ENPP1 (Ecto-nucleotide pyrophosphatase phosphodiesterase 1) is a type II transmembrane glycoprotein originally identified as a negative regulator of bone mineralization. ENPP1 is expressed on the cell surface in mineralizing cells, such as osteoblasts and chondrocytes, and hydrolyzes extracellular ATP to produce AMP and diphosphate, an inhibitor of bone mineralization. A recent study reported that ENPP1 also hydrolyzes 2′3′-cGAMP, but not 3′3′-cGAMP, and negatively regulates the cGAS-STING-dependent immune activation. Here, we report the crystal structures of ENPP1 in complex with 3′3′-cGAMP and the reaction intermediate pA(3′,5′)pG (pApG).

We co-crystallized the ENPP1-ΔSMB T238A mutant in the presence of 2′3′-cGAMP or 3′3′-cGAMP, and determined the crystal structures at 1.8 and 1.9 Å resolutions, respectively. In the co-crystal structure with 2′3′-cGAMP, a continuous density was not observed at the 2′-5′ phosphodiester linkage of 2′3′-cGAMP, suggesting that 2′3′-cGAMP was predominantly degraded to the pApG linear intermediate during crystallization, although the catalytically inactive ENPP1-ΔSMB T238A mutant was used for crystallization. This may be due to the slight enzymatic activity of the mutant at a high concentration during crystallization. We concluded that this structure represents a post-reaction state of the first hydrolysis, and modeled pApG into the electron density. pApG adopts an open conformation, in which the nucleobases are far apart from each other. The adenine and guanine moieties of pApG are accommodated within the nucleotide-binding pocket (N-pocket) and the guanine-binding pocket (G-pocket), respectively. The 5′-phosphate group binds to two zinc ions (Zn1 and Zn2), which are coordinated by Asp358/His362/His517 and Asp200/Asp405/His406, respectively. This observation suggests that ENPP1 first hydrolyzes the 2′-5′, rather than the 3′-5′, phosphodiester linkage in 2′3′-cGAMP, consistent with previous data showing that a 2′3′-cGAMP analog with the 2′-5′ non-hydrolyzable phosphothioate diester linkage (2′3′-cGAsMP) is not degraded by ENPP123. The guanosine moiety of pApG is accommodated in the G-pocket, formed by His362 on a short helix and a loop (residues 510–517). The 3′-OH group of the guanosine forms a hydrogen bond with Asn259, while the guanine base is stacked with His362, with its N1 atom forming a hydrogen bond with Ser514.

> GPKSWVEETCESIDTPECPAEFESPPTLLFSLDGFRAEYLHTWGGLLPVISKLKNCGTYTKNMRPMYPTKAFPNHYSIVTGLYPESHGIIDNKMYDPKMNASFSLKSKEKFNPLWYKGQPIWVTANHQEVKSGTYFWPGSDVEIDGILPDIYKVYNGSVPFEERILAVLEWLQLPSHERPHFYTLYLEEPDSSGHSHGPVSSEVIKALQKVDRLVGMLMDGLKDLGLDKCLNLILISDHGMEQGSCKKYVYLNKYLGDVNNVKVVYGPAARLRPTDVPETYYSFNYEALAKNLSCREPNQHFRPYLKPFLPKRLHFAKSDRIEPLTFYLDPQWQLALNPSERKYCGSGFHGSDNLFSNMQALFIGYGPAFKHGAEVDSFENIEVYNLMCDLLGLIPAPNNGSHGSLNHLLKKPIYNPSHPKEEGFLSQCPIKSTSNDLGCTCDPWIVPIKDFEKQLNLTTEDDDIYHMTVPYGRPRILLKQHRVCLLQQQQFLTGYSLDLLMPLWASYTFLSNDQFSRDDFSNCLYQDLRIPLSPVHKCSYYKSNSKLSYGFLTPPRLNRVSNHIYSEALLTSNIVPMYQSFQVIWHYLHDTLLQRYAHERNGINVVSGPVFDFDYDGRYDSLEILKQNSRVIRSQEILIPTHFFIVLTSCKQLSETPLECSALESSAYILPHRPDNIESCTHGKRESSWVEELLTLHRARVTDVELITGLSFYQDRQESVSELLRLKTHLPIFSQED>[2x]GGUCACA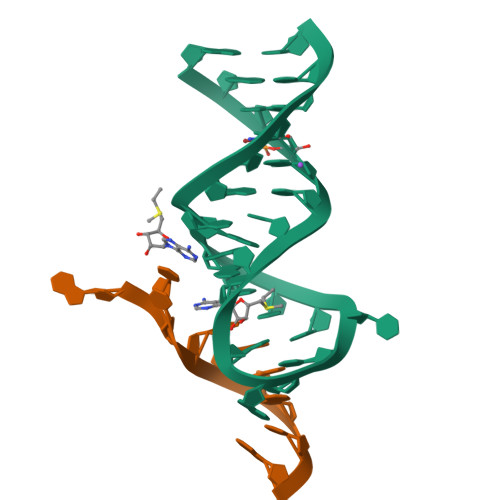ACGGCUUCCUGGCGUGACC;>AUUGGAGCA[2x]> GCCSLPPCALNN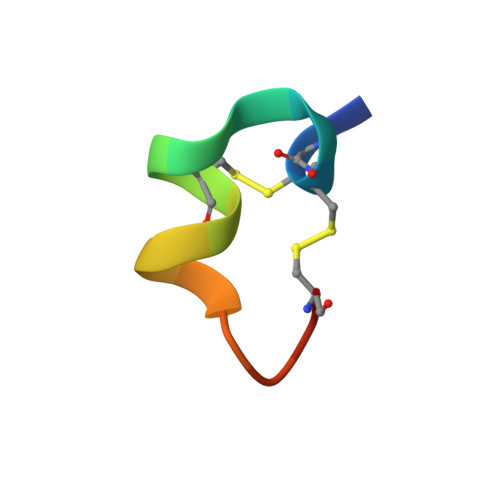PKYCX> MSEESQAFQRQLTALIGYDVTDVSNVHDDELEFTRRGLVTPRMAEVASRDPKLYAMHPWVTSKPLPEYLWKKIANNCIFIVIHRSTTSQTIKVSPDDTPGAILQSFFTKMAKKKSLMDIPESQSEQDFVLRVCGRDEYLVGETPIKNFQWVRHCLKNGEEIHVVLDTPPDPALDEVRKEEWPLVDDCTGVTGYHEQLTIHGKDHESVFTVSLWDCDRKFRVKIRGIDIPVLPRNTDLTVFVEANIQHGQQVLCQRRTSPKPFTEEVLWNVWLEFSIKIKDLPKGALLNLQIYCGKAPALSSKASAESPSSESKGKVQLLYYVNLLLIDHRFLLRRGEYVLHMWQISGKGEDQGSFNADKLTSATNPDKENSMSISILLDNYCHPIALPKHQPTPDPEGDRVRAEMPNQLRKQLEAIIATDPLNPLTAEDKELLWHFRYESLKHPKAYPKLFSSVKWGQQEIVAKTYQLLARREVWDQSALDVGLTMQLLDCNFSDENVRAIAVQKLESLEDDDVLHYLLQLVQAVKFEPYHDSALARFLLKRGLRNKRIGHFLFWFLRSEIAQSRHYQQRFAVILEAYLRGCGTAMLHDFTQQVQVIEMLQKVTLDIKSLSAEKYDVSSQVISQLKQKLENLQNSQLPESFRVPYDPGLKAGALAIEKCKVMASKKKPLWLEFKCADPTALSNETIGIIFKHGDDLRQDMLILQILRIMESIWETESLDLCLLPYGCISTGDKIGMIEIVKDATTIAKIQQSTVGNTGAFKDEVLNHWLKEKSPTEEKFQAAVERFVYSCAGYCVATFVLGIGDRHNDNIMITETGNLFHIDFGHILGNYKSFLGINKERVPFVLTPDFLFVMGTSGKKTSPHFQKFQDICVKAYLALRHHTNLLIILFSMMLMTGMPQLTSKEDIEYIRDALTVGKNEEDAKKYFLDQIEVCRDKGWTVQFNWFLHLVLGIKQGEKHSA

Phosphoinositide 3-kinases (PI3Ks) promote cell growth, survival, division and motility, and signal through protein kinase B (PKB/Akt) and the mammalian target of rapamycin (mTOR) to control cellular growth and proliferation. BKM120 is a potent PI3K inhibitor, but has been reported to also act as a microtubule-destabilizing agent (MDA). We succeeded in separating the activities of BKM120 as a PI3K inhibitor and an MDA by minimal chemical modification of its core pyrimidine ring.

A 3.2 Å resolution crystal structure of the PI3Kγ catalytic subunit (p110γ) in complex with BKM120 has been previously reported. At this resolution a precise positioning of the BKM120 molecule in the p110γ-binding site is not possible. To validate the rotational orientation of BKM120 in PI3K, the asymmetrically substituted BKM120 derivatives PIKiN1 and PIKiN2, as well as their relevant regioisomers PIKiN1-R1 and PIKiN2-R1, were produced. Interestingly, PIKiN1 and PIKiN2 bound to recombinant p110γ, p110α, p110β and p110δ with a 7–30-fold higher affinity as compared to their regioisomers, which was also confirmed in a p110α activity assay measuring directly PtdIns(3,4,5)P3. To clearly determine the orientation of the substituted morpholino group, a bulky chloromethyl-azetidin-methanol substitution was introduced: here the orientation of the pyrimidine core of PIKiN2 bound to p110γ could be unambiguously determined in a crystal structure resolved to 2.51 Å. Its core pyrimidine C–H group points towards Tyr867 (position U in Fig. 5e and Supplementary Table 8). Closer inspection of the p110γ–PI3KiN2 and p110γ–PI3KiN3 complex structures revealed that (i) the core nitrogen in position V is hydrogen bonded through a structured water molecule to Asn951 and Asp964, and (ii) that the trifluoromethyl-pyridin-2-amine group and aspartates 841, 836, 964 coordinate two additional structured water molecules (best resolved in the PI3KiN3 complex). Molecular dynamics simulations with BKM120 docked into p110γ demonstrated that positioning of the pyrimidine core C–H group towards Tyr867 kept the structured water network intact (CU–H). In contrast, when BKM120 was oriented as in the initially reported structure by Burger and colleagues (CV–H), hydrogen bond interactions between the inhibitor, water molecules, side chains of Asp964 and Asp836 were disrupted.> MNINQLILRNLKKNLRNYYLYVFALIFSVALYFAFVTLQYDPAINEVKASIKGAAAIKTASILLVAVVAIFILYANTIFIKRRSKEIGLFQLIGMTKHKIFRILSAENVMLYFGSLAIGVAAGFSISKLVLMILFKIVDVKADAKLHFSEQALVQTVIVFCGIYLLIMIMNYTFIKKQSILSLFKVTSSTEDKVKKISFFQMLIGALGIVLILTGYYVSSELFGGKFKTINELFVAMSFILGSVIIGTFLFYKGSVTFISNIIRKSKGGYLNISEVLSLSSIMFRMKSNALLLTIITTVSALAIGLLSLAYISYYSSEKTAEQNVAADFSFMNEKDAKLFENKLRESNISFVKKATPVLQANVDIANIMDGTPKEMQGDPGNMQLAVVSDKDVKGVDVAAGEAVFSGYTDLLQKIMVFKDSGVIKVKSKHETQPLKYKGLREEFLVSYTFTSGGMPAVIVDDSLFKQLDKDKDPRIQLAQSTFIGVNVKHDDQMEKANELFQQVNKKNEHLSRLDTSAAQKSLFGMVMFIVGFLGLTFLITSGCILYFKQMGESEDEKPSYTILRKLGFTQGDLIKGIRIKQMYNFGIPLVVGLFHSYFAVQSGWFLFGSEVWAPMIMVMVLYTA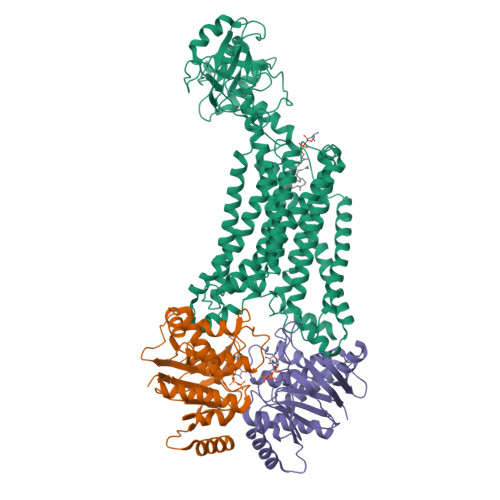LYSIFGFLSVLYYKKVIKSSL;>MSGHHHHHHVILEANKIRKSYGNKLNKQEVLKGIDIHIEKGEFVSIMGASGSGKTTLLNVLSSIDQVSHGTIHINGNDMTAMKEKQLAEFRKQHLGFIFQDYNLLDTLTVKENILLPLSITKLSKKEANRKFEEVAKELGIYELRDKYPNEISGGQKQRTSAGRAFIHDPSIIFADQPTGALDSKSASDLLNKLSQLNQKRNATIIMVTHDPVAASYCGRVIFIKDGQMYTQLNKGGQDRQTFFQDIMKTQGVLGGVQHEH[2x]>[2x]GPHMSDHKFLTQAVEEAYKGVDCGDGGPFGAVIVHNNEVVASCHNMVLKYTDPTAHAEVTAIREACKKLNKIELSECEIYASCEPCPMCFGAIHLSRLKRLVYGAKAEAAIAIGFDDFIADALRGTGVYQKSSLEIKKADGNGAAIAEQVFQNTKEKFRLY

In plants, guanosine deaminase (GSDA) catalyzes the deamination of guanosine for nitrogen recycling and re-utilization. The other involves the hydrolysis of Gua to guanine (G), followed by its deamination to xanthine under the action of guanine deaminase (GDA). Both deaminases are zinc-dependent enzymes, which rely on a catalytic water molecule to attack the amino group-connecting C2 atom to proceed with the catalysis. The zinc ions are tightly bound to the active site, coordinated by the completely conserved residues His80, Cys113, Cys110, and the key water molecule. AtGSDA catalysis needs two key sub-processes: the activation of water and re-capping of the active site, which proceed via the two critical residues Glu82 and Tyr185, respectively.

Despite its reported strict specificity toward Gua only, we managed to identify that 2′-O-methylguanosine (2′-O-mG) and N2-methylguanosine (N2-mG) could be employed as reasonable substrates of AtGSDA by testing a series of Gua derivatives, but the structural basis is unclear. Besides the rapid conversion of the natural substrate, the other two substrates were almost completely converted as well, because their planar purine rings almost coincided with that of Xan bound by AtGSDA. Interestingly, 2′-O-mG was different from the canonical Gua binding mode in that its ribose ring flips ~180°, which brought the 5′-hydroxyl to the vicinity of Tyr185 and formed hydrogen bonds with its carboxylate group; however, the ribose lost the contact with the mainchain of Asn140 instead. The results indicated that the starting material Gua in a reaction would completely disappear in 2 h, while only ~15% 2′-O-mG or very little N2-mG was converted into the product. By the 24-h time point, the 2′-O-mG reaction would almost finish while the majority of N2-mG was still in the substrate form. We found that the product Xan and 2′-O-mG would boost the Tm value by nearly 2 °C, which may be related to the unusual binding mode. The fact that 2′-O-mX could be efficiently bound by a non-canonical mode and acted upon suggested that the binding pocket of AtGSDA still has room for alternative binding possibilities. Actually, according to DoGSiteScorer, the 2′-O-mG-bound AtGSDA had a slightly larger pocket than the Xan-bound AtGSDA, suggesting the moderate plasticity of the binding pocket of the enzyme.>STAGKVIKCKAAVLWEEKKPFSIEEVEVAPPKAHEVRIKMVATGICRSDDHVVSGTLVTPLPVIAGHEAAGIVESIGEGVTTVRPGDKVIPLFTPQCGKCRVCKHPEGNFCLKNDLSMPRGTMQDGTSRFTCRGKPIHHFLGTSTFSQYTVVDEISVAKIDAASPLEKVCLIACGFSTGYGSAVKVAKVTQGSTCAVFGLGGVGLSVIMGCKAAGAARIIGVDINKDKFAKAKEVGATECVNPQDYKKPIQEVLTEMSNGGVDFSFEVIGRLDTMVTALSCCQEAYGVSVIVGVPPDSQNLSMNPMLLLSGRTWKGAIFGGFKSKDSVPKLVADFMAKKFALDPLITHVLPFEKINEGFDLLRSGESIRTILTF[2x]

Horse liver alcohol dehydrogenase catalyzes hydrogen transfer with quantum-mechanical tunneling that involves fast motions in the active site. The catalytic and coenzyme-binding domains are connected by a hinge region that was identified by comparing the structure of the open conformation of the apoenzyme with the closed holoenzyme, where a rotation of about 10° closes the cleft between the domains where the substrates bind. The O atoms of the alcohols are ligated to the catalytic zinc at a distance expected for a zinc alkoxide (1.97 Å) and participate in a low-barrier hydrogen bond (2.52 Å) to the hydroxyl group of Ser48 in the proton-relay system.

The G173A mutant enzyme was also studied because the substitution in the hinge region could affect the conformational change, even though the steady-state kinetic constants are very similar to those for the wild-type enzyme and the X-ray structure shows that the methyl group of Ala173 is accommodated in a pre-existing cavity. In the present study, the temperature dependence of B factors was determined by X-ray crystallography of three ternary complexes of horse liver alcohol dehydrogenase from 25 to 85 K with a helium cryostat and from 100 to 150 K with a nitrogen cryostat. The mounting stems were stabilized with expoxy glue for the G173A ADH crystals, but this did not seem to affect the mosaicity or the B factors as a function of temperature in the different cryostreams. In contrast, crystallization with fluorinated alcohols inhibits the reduction of NAD+ to NADH, and the NAD+ and the alcohols in the complexes are positioned appropriately for direct hydride transfer, with the pro-R hydrogen of the methylene C atom pointing towards C4N of the nicotinamide ring of the coenzyme at a distance of 3.4–3.5 Å. The B factors for the crystals with PFB were larger than those with TFE, suggesting that the crystal quality is a factor. The overall and residual B factors for the protein, C4N of NAD+ and the methylene C atom of the alcohol obtained by TLS refinement are almost temperature independent.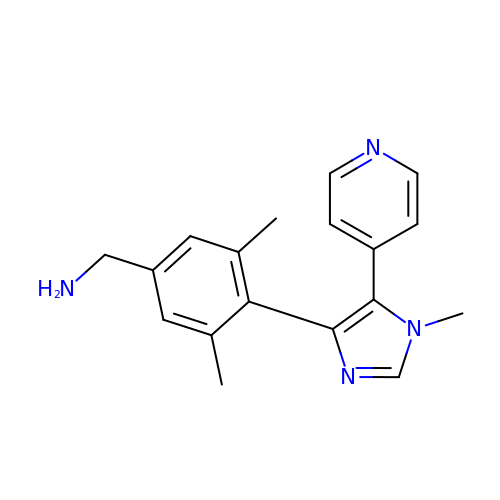[3,5-dimethyl-4-(1-methyl-5-pyridin-4-yl-imidazol-4-yl)phenyl]methanamine | C18 H20 N4 | LYFZPAXTPPYSEC-UHFFFAOYSA-N>AIAHLATEYVFSDFLLKEPTEPKFKGLRLELAVDKMVTCIAVGLPLLLISLAFAQEISIGTQISCFSPSSFSWRQAAFVDSYCWAAVQQKNSLQSESGNLPLWLHKFFPYILLLFAILLYLPPLFWRFAAAPHICSDLKFIMEELDKVY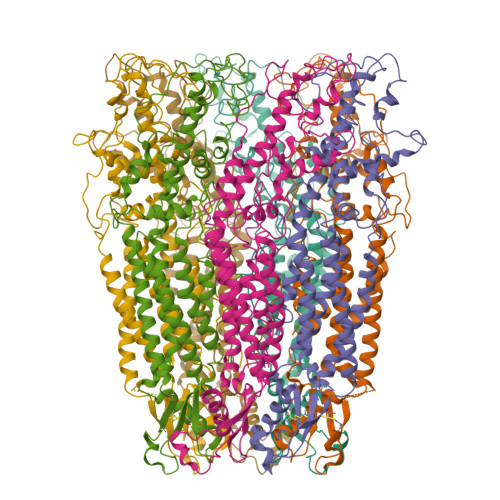NRAIKAAKSARDLDMRDGACSVWSHPQFEKPGVTENLGQSLWEVSESHFKYPIVEQYLKTKKNSNNLIIKYISCRLLTLIIILLACIYLGYYFSLSSLSDEFVCSIKSGILRNDSTVPDQFQCKLIAVGIFQLLSVINLVVYVLLAPVVVYTLFVPFRQKTDVLKVYEILPTFDVLHFKSEGYNDLSLYNLFLEENISEVKSYKCLKVLENIKSSGQGIDPMLLLTNLGMIKMDVVDGKTPMSAEMREEQGNQTAELQGMNIDSETKANNGEKNARQRLLDSSC[7x]>[2x]GESWQKRYDSLQKIVEKQQQKMDQLRSQVQSLEQEVAQEEGTSQALREE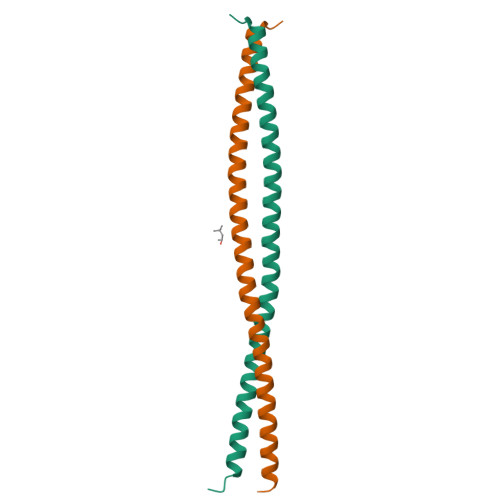AQRRDSALQQLRTAVKELSVQNQDLIEKNLTLQEHLRQA> GSEFMTEAALVEGQVKLRDGKKWKSRWLVLRKPSPVADCLLMLVYKDKCERSK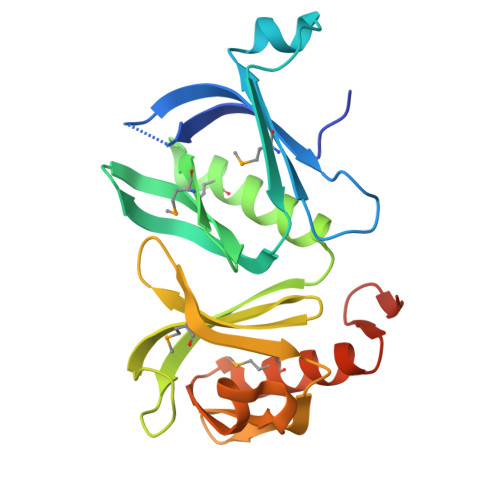GLRERSSLTLEDICGLEPALPYEGLAHTLAIICLSQAVMLGFDSHEAMCAWDTRIRYALGEVHRFHVTVAPGTKLESGPATLHLCNDILVLARDIPPTVMGQWKLSDLRRYGAVPNGFIFEGGTRCGYWAGVFFLSSAEGEQMSFLFDCIVRGISPTKGPFGLRPVLPDPS Transcription activator-like effectors (TALEs) compose a family of virulence proteins that act as transcriptional activator factors in plant cells. TALEs are organized into three different domains: an N-terminal region involved in protein translocation by the bacterial secretion system, a central DNA-binding domain and a C-terminal region that contains both the nuclear localization signal sequence and an acidic transcriptional activation region. The central DNA-binding domain is composed of an array of tandem repeats which recognizes the DNA target. The DNA bases recognized by each repeat are specified by the amino-acid sequence of the RVDs, establishing a direct code between these pairs of amino acids in each repeat and the nucleotides in the target sequence.

Here, we present the crystal structure of the DNA-binding region of AvrBs3 from Xanthomonas campestris bound to its target sequence present in the pepper Bs3 promoter, including the N-terminal region interacting with the initial thymine. The model was refined to 2.55 Å resolution. However, the quality of the electron density is excellent from the first repeat until the middle of repeat 17 in residue 830; in the N-terminal region the electron density is defined such that side chains can be observed from residue 230 onwards. The protein shows a left-handed packing of the consecutive helices within and between the individual repeats. The sequence-specific contacts of TALE AvrBs3 with the DNA are exclusively made by the residue at position 13 in each RVD interacting with the corresponding base on the sense strand. In contrast, the side chain of the residue at position 12 of each RVD contacts the backbone carbonyl O atom at position 8 in each repeat, constraining the RVD-containing loop. The AvrBs3–DNA structure displays seven HD RVDs. The HD RVD contacting A1 displays a hydrogen bond (3.01 Å) between the side chain of Asp301 in the first RVD and the NH2 group of the base. The side chains of these residues converge near the adjacent T−1 and T0 bases, contacting the methyl groups of these bases through van der Waals interactions. Moreover, the side chains of Thr270, Gln305 and Gly267 are involved in a network of hydrogen bonds surrounding the phosphate of T0.

> VDLRTLAYSQQQQEKIKPKVRSTVAQHHEALVAHAFTHAHIVALSQHPAALATVAVKYQDMIAALPEATHEAIVAVAKQWSGARALEALLTVAGELRGPPLQLDTGQLLKIAKRGGVTAVEAVHAWRNALTGAPLNLTPEQVVAIASHDGGKQALETVQRLLPVLCQAHGLTPQQVVAIASNGGGKQALETVQRLLPVLCQAHGLTPEQVVAIASNIGGKQALETVQALLPVLCQAHGLTPQQVVAIASNGGGKQALETVQRLLPVLCQAHGLTPEQVVAIASNIGGKQALETVQALLPVLCQAHGLTPEQVVAIASNIGGKQALETVQALLPVLCQAHGLTPEQVVAIASNIGGKQALETVQALLPVLCQAHGLTPEQVVAIASHDGGKQALETVQRLLPVLCQAHGLTPEQVVAIASHDGGKQALETVQRLLPVLCQAHGLTPQQVVAIASNGGGKQALETVQRLLPVLCQAHGLTPEQVVAIASNIGGKQALETVQALLPVLCQAHGLTPEQVVAIASNIGGKQALETVQALLPVLCQAHGLTPEQVVAIASHDGGKQALETVQRLLPVLCQAHGLTPEQVVAIASHDGGKQALETVQRLLPVLCQAHGLTPEQVVAIASHDGGKQALETVQRLLPVLCQAHGLTPQQVVAIASNGGGKQALETVQRLLPVLCQAAGLTPEQVVAIASHDGGKQALETVQRLLPVLCQAHGLTPQQVVAIASNGGGRPALESIVAQLSRPDPGSSAALEHHHHHH>[4x]GSDPQVLRGSGHCKWFNVRMGFGFISMTSREGSPLENPVDVFVHQSKL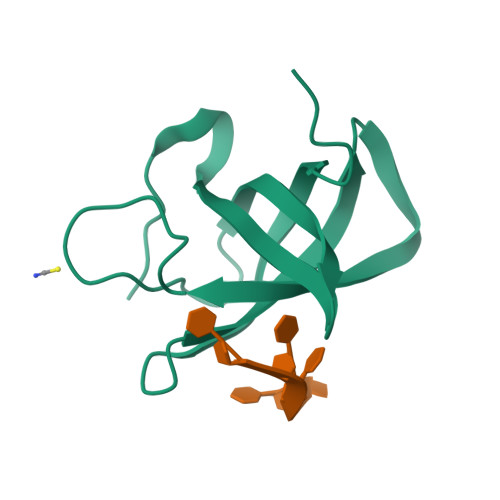YMEGFRSLKEGEPVEFTFKKSSKGFESLRVTGPGGNPCLGNE(3S)-3,7-diaminoheptan-2-one 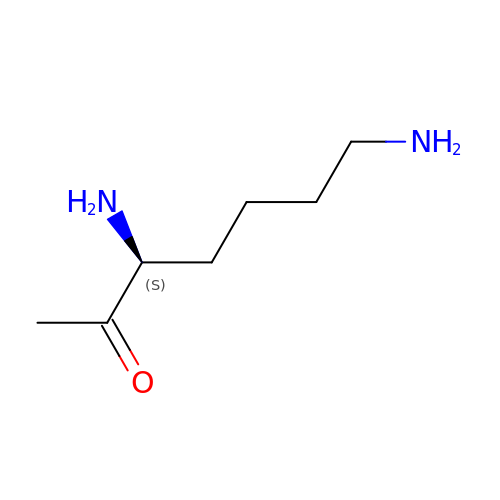| C7 H16 N2 O | FADKJNSSIWTVAI-ZETCQYMHSA-N> IVGGKVCPKGECPWQVLLLVNGAQLCGGTLINTIWVVSAAHCFDKIKNWRNLIAVLGEHDLSEHDGDEQSRRVAQVIIPSTYVPGTTNHDIALLRLHQPVVLTDHVVPLCLPERTFSERTLAFVRFSLVSGWGQ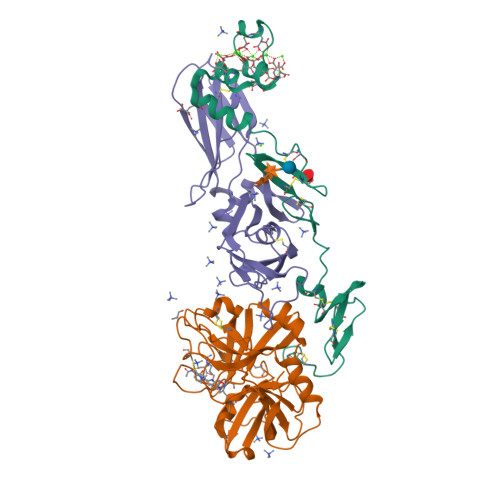LLDRGATALELMVLNVPRLMTQDCEASFPGKITEYMFCAGYSDGSKDSCKGDSGGPHATHYRGTWYLTGIVSWGQGCATVGHFGVYTRVSQYIEWLQKLMRSEPRPGVLLRAPFP;> ANAFLEELRPGSLERECKEEQCSFEEAREIFKDAERTKLFWISYSDGDQCASSPCQNGGSCKDQLQSYICFCLPAFEGRNCETHKDDQLICVNENGGCEQYCSDHTGTKRSCRCHEGYSLLADGVSCTPTVEYPCGKIPILEKRNASKPQGR;> SGTTNTVAAYNLTWKSTNFKTILEWEPKPVNQVYTVQISTKSGDWKSKCFYTTDTECDLTDEIVKDVKQTYLARVFSYPAGNVESTGSAGEPLYENSPEFTPYLETNLGQPTIQSFEQVGTKVNVTVEDERTLVRRNNTFLSLRDVFGKDLIYTLYYWKSSSSGKKTAKTNTNEFLIDVDKGENYCFSVQAVIPSRTVNRKSTDSPVECMGQEKGEFRE>[2x]MATNNNQIGENKEQTIFDHKGNVIKTEDREIQIISKFEEPLIVVLGNVLSDEECDELIELSK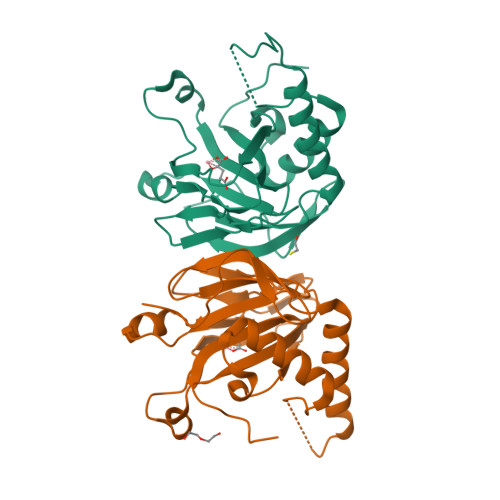SKLARSKVGSSRDVNDIRTSSGAFLDDNELTAKIEKRISSIMNVPASHGEGLHILNYEVDQQYKAHYDYFAEHSRSAANNRISTLVMYLNDVEEGGETFFPKLNLSVHPRKGMAVYFEYFYQDQSLNELTLHGGAPVTKGEKWIATQWVRRGTYKPPGPPGPPG> QISQAI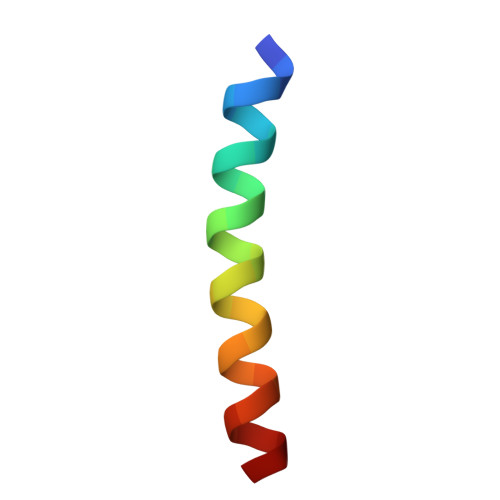KYLQNNIKGFIIRQRVNDE> GPGYQDPARSVRHIAIPAHRGLITDRNGEPLAVSTPVTTLWANPKELMTAKERWPQLAAALGQDTKLFADRIEQNAEREFIYLVRGLTPEQGEGVIALKVPGVYSIEEFRRFYPAGEVVAHAVGFTDVDDRGREGIELAFDEWLAGVPGKRQVLKDRRGRVIKDVQVTKNAKPGKTLALSIDLRLQYLAHRELRNALLENGAKAGSLVIMDVKTGEILAMTNQPTYNPNNRRNLQPAAMRNRAMIDVFEPGSTVKPFSMSAALASGRWKPSDIVDVYPGTLQIGRYTIRDVSRNSRQLDLTGILIKSSNVGISKIAFDIGAESIYSVMQQVGLGQDTGLGFPGERVGNLPNHRKWPKAETATLAYGYGLSVTAIQLAHAYAALANDGKSVPLSMTRVDRVPDGVQVISPEVASTVQGMLQQVVEAQGGVFRAQVPGYHAAGKSGTARKVSVGTKGYRENAYRSLFAGFAPATDPRIAMVVVIDEPSKAGYFGGLVSAPVFSKVMAGALRL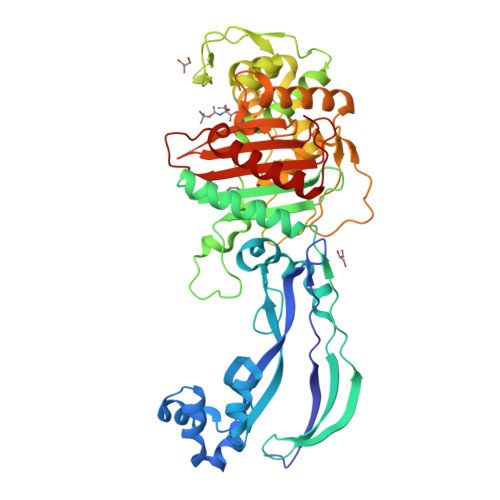MNVPPDNLPTA Phosphoglucomutase (EC 5.4.2.2., PGM), a key enzyme of glycogenolysis and glycogenesis, catalyzes the interconversion of glucose 1-phosphate and glucose 6-phosphate, whereas phosphomannomutase (EC 5.4.2.8., PMM) transfers the phosphate group from the 1′ to the 6′, or from the 6′ to the 1′ position in mannose phosphate. However, in the hyperthermophilic archaeon Thermococcus kodakarensis, a single gene, Tk1108, encodes a protein with both PGM and PMM activities. Among the remaining three gene products, only that of Tk1108 exhibited both phosphoglucomutase and phosphomannomutase activities; based on its former function, the protein was named PGMTk. Moreover, thermostability studies confirmed a half-life of 85 min at 100 °C.

The map of PGMTk was determined at a nominal resolution of 2.45 Å with D2 symmetry, as shown by the GSFSC plot (FSC = 0.143). The tetrameric structure of PGMTk is constituted of two dimers arranged in D2 symmetry. The structural analysis of the protomers in the tetramer display no significant deviations in the conformation. Alignment of 453 residues of chain A to those of chains B, C, and D using GESAMT resulted in root mean square deviation (RMSD) values of 0.18, 0.18, and 0.17 Å, respectively. The protomer of PGMTk exhibited a three-layer α-β-α sandwich architecture with a unique α/β topology and arrangement. Residues 3–138 constitute domain I, residues 156–256 form domain II, residues 261–370 comprise domain III, and residues 384–443 account for domain IV or the C-terminal domain. The first three domains adopt a three-layer α/β/α sandwich architecture, whereas domain IV or the C-terminal domain form a two-layer α/β sandwich topology. In PGMTk, the N- and C-terminal regions adopt a compact, nearly perpendicular orientation, with an interdomain angle of 95.7°. The N-terminal domain was found to have lower B-factors and showed a rigid symmetry, while the flexible C-terminal region had comparatively larger B-factors. The alignment of PGMTk structures predicted by AlphaFold2 and experimentally obtained using cryo-EM showed an RMSD of only 0.41 Å.

>MGKLFGTFGVRGIANEEITPEFALKIGMAFGTLLKREGRERPLVVVGRDTRVSGEMLKDALISGLLSTGCDVIDVGIAPTPAIQWATNHFNADGGAVITASHNPPEYNGIKLLEPNGMGLKKEREAIVEELFFSEDFHRAKWNEIGELRKEDIIKPYIEAIKNRVDVEAIKKRRPFVVVDTSNGAGSLTLPYLLRELGCKVVSVNAHPDGHFPARNPEPNEENLKGFMEIVKALGADFGVAQDGDADRAVFIDENGRFIQGDKTFALVADAVLRENGGGLLVTTIATSNLLDDIAKRNGAKVMRTKVGDLIVARALLENNGTIGGEENGGVIFPDFVLGRDGAMTTAKIVEIFAKSGKKFSELIDELPKYYQFKTKRHVEGDRKAIVAKVAELAEKKGYKIDTTDGTKIIFDDGWVLVRASGTEPIIRIFSEAKSEEKAREYLELGIKLLEEALKG[4x]> DGIIDNAQDNVNATLKSLTKQYLSVSNSID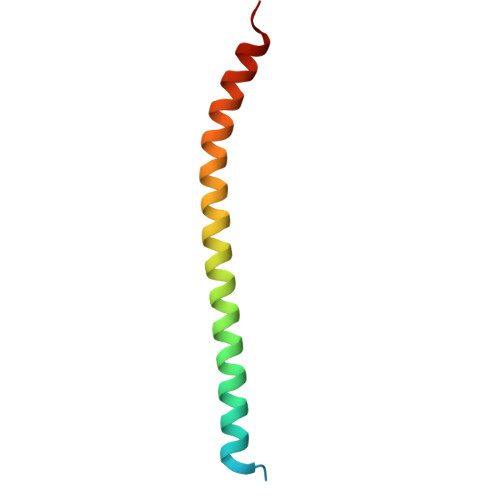ETVARYKAQFTQLDTMMSKLNNTSSYLTQQFTAMNKS>[2x]GTLTGERPPVFWLQGQGCTGCSVTLLNSVHPSIADVLLKVISLEFHPTVMAWEGEHAIEHMRKVAEKFKGKFFLVIEGSVPVEADGKYCIIGEANHHEISMVDALKEFGPNAAAVLAVGTCAAYGGIPAAEGSETGATAVSKFLGDNGIKTPVVNIPGCPPHPDWIVGTVVLALDAIKKNGLEGGLAEVVKVLDSDGRPTPFFGRNIHENCPYLDKYDEGVMSATFTDKVGCRYDLGCKGPMTMADCFERKWNGGVNWCVQNAVCIGCVEPDFPDGKSPFYQA;>[2x]GATGRTTIAIDPVTRIEGHLKAEVVVENGKVVDARLSGGMYRGFETILRGRDPRDASQIVQRICGVCPTAHSTASVLALDEAFGAKVPNNGRITRNLIFGANYLQSHILHFY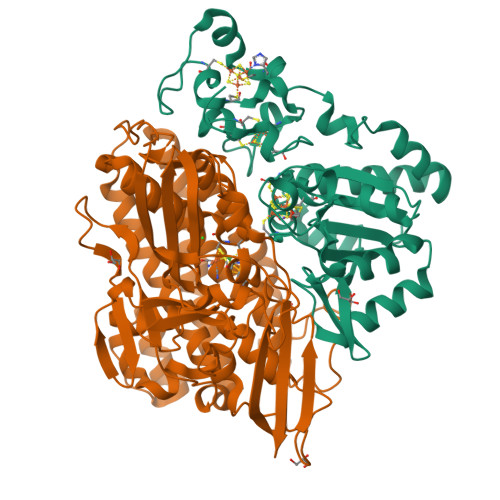HLSAQDFVQGPDTAPFVPRFPKSDLRLSKELNKAGVDQYIEALEVRRICHEMVALFGGRMPHVQGQVVGGATEIPTKEKLVEYAARFKKVRDFVEQKYVPVVYTIGSKYKDMFKVGQGFKAALCVGAFPLDNSGKKHLFMPGVYAKGKDMPFDPSKIKEYVKYSWFAEETTGLNYKEGKTIPAPDKAGAYSFVKAPRYDGLSLEVGPLARMWVNNPELSPVGKKLLKDLFGISAKKFRDLGEEAAFSLMGRHVARAEETYYMLGAIEGWLKEIKAGEDTVVMPAVPASAEGTGFTEAPRGSLLHYVKVKDSKIDNYQIVSASLWNCNPRDDMGQRGAVEEALIGIPVDDIQNPVNVARLIRAFDPULGCAVH>[4x]TKLNGMVLLCKVCGD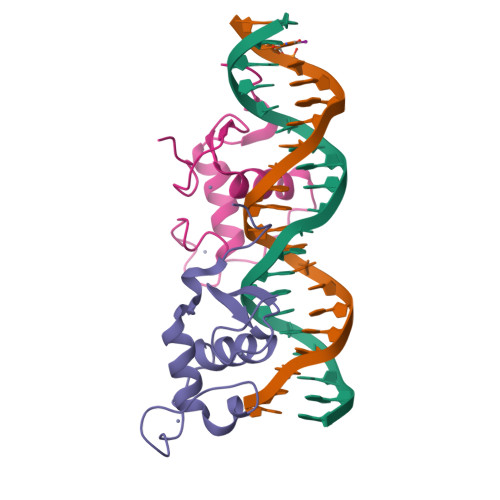VASGFHYGVLACEGCKGFFRRSIQQNIQYKRCLKNENCSIVRINRNRCQQCRFKKCLSVGMSRDAVRFGRIPKREKQRM methyl L-phenylalaninate 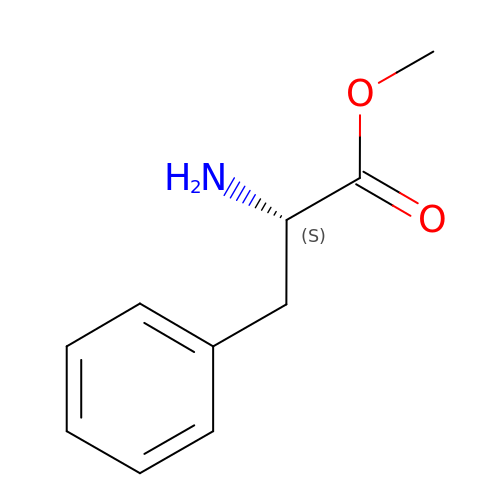| C10 H13 N O2 | VSDUZFOSJDMAFZ-VIFPVBQESA-N4-[2-[2-hydroxyethyl(phenyl)amino]-2-oxidanylidene-ethyl]-~{N}-oxidanyl-benzamide | C17 H18 N2 O4 | 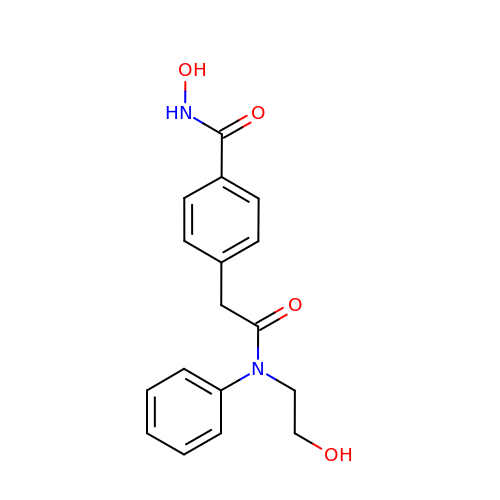RFAZNTABYJYOAR-UHFFFAOYSA-N> QANLMRLKSDLFNRSPMYPGPTKDDPLTVTLGFTLQDIVKVDSSTNEVDLVY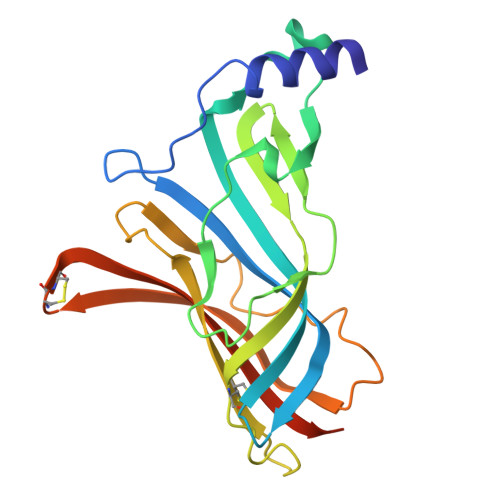YEQQRWKLNSLMWDPNEYGNITDFRTSAADIWTPDITAYSSTRPVQVLSPQIAVVTHDGSVMFIPAQRLSFMCDPTGVDSEEGVTCAVKFGSWVYSGFEIDLKTDTDQVDLSSYYASSKYEILSATQTRQVQHYSCCPEPYIDVNLVVKFRERRAGNGFFRNLFD> GPLGSAGKSSLFKIILLGDGGVGKSSLMNRYVTNKFDSQLFHTIGVEFLNKDLEVDGHFVTMQIWDTAGQERFRSLRTPFYRGSDCCLLTFSVDDSQSFQNLSNWKKEFIYYADVKEPESFPFVILGNKTDIKERQVSTEEAQAWCKDNGDYPY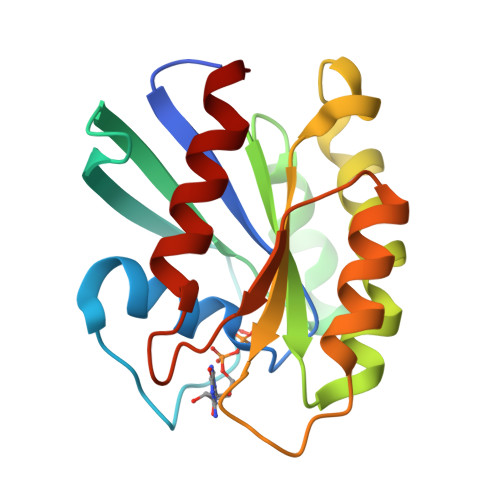FETSAKDSTNVAAAFEEAVRRILAT(4R)-6-[(2,5-dichloro-3-{[(2R,4R)-1-(cyclopentanecarbonyl)-2-methylpiperidin-4-yl]oxy}phenyl)amino]-6-oxo-4-phenylhexanoic acid | C30 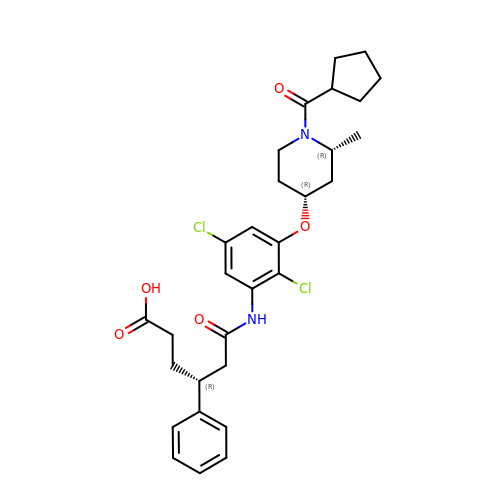H36 Cl2 N2 O5 | NWXXXIQTJWEGQR-ZFJSRUIDSA-N N~2~-[4-cyano-3-(trifluoromethyl)phenyl]-N,N-dimethyl-N~2~-(2,2,2-trifluoroethyl)-L-alaninamide | C15 H15 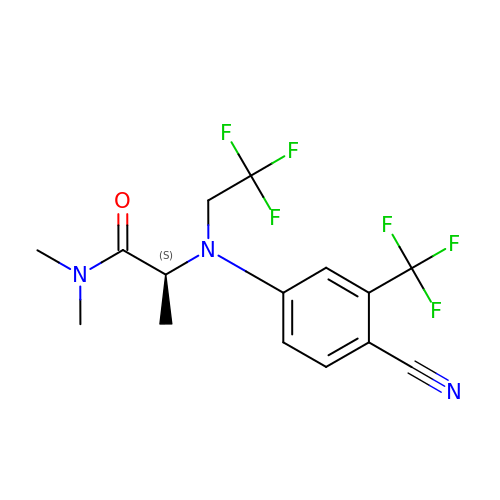F6 N3 O | BEFAEFLFXOZVJY-VIFPVBQESA-N> MSADSSPLVGSTPTGYGTLTIGTSIDPLSSSVSSVRLSGYCGSPWRVIGYHVVVWMMAGIPLLLFRWKPLWGVRLRLRPCNLAHAETLVIEIRDKEDSSWQLFTVQVQTEAIGEGSLEPSPQSQAEDGRSQAAVGAVPEGAWKDTAQLHKSEEAVSVGQKRVLRYYLFQGQRYIWIETQQAFYQVSLLDHGRSCDDVHRSRHGLSLQDQMVRKAIYGPNVISIPVKSYPQLLVDEALNPYYGFQAFSIALWLADHYYWYALCIFLISSISICLSLYKTRKQSQTLRDMVKLSMRVCVCRPGGEEEWVDSSELVPGDCLVLPQEGGLMPCDAALVAGECMVNESSLTGESIPVLKTALPEGLGPYCAETHRRHTLFCGTLILQARAYVGPHVLAVVTRTGFCTAKGGLVSSILHPRPINFKFYKHSMKFVAALSVLALLGTIYSIFILYRNRVPLNEIVIRALDLVTVVVPPALPAAM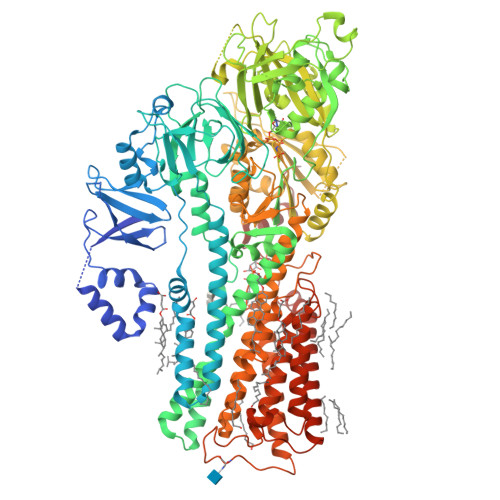TVCTLYAQSRLRRQGIFCIHPLRINLGGKLQLVCFDKTGTLTEDGLDVMGVVPLKGQAFLPLVPEPRRLPVGPLLRALATCHALSRLQDTPVGDPMDLKMVESTGWVLEEEPAADSAFGTQVLAVMRPPLWEPQLQAMEEPPVPVSVLHRFPFSSALQRMSVVVAWPGATQPEAYVKGSPELVAGLCNPETVPTDFAQMLQSYTAAGYRVVALASKPLPTVPSLEAAQQLTRDTVEGDLSLLGLLVMRNLLKPQTTPVIQALRRTRIRAVMVTGDNLQTAVTVARGCGMVAPQEHLIIVHATHPERGQPASLEFLPMESPTAVNGVKDPDQAASYTVEPDPRSRHLALSGPTFGIIVKHFPKLLPKVLVQGTVFARMAPEQKTELVCELQKLQYCVGMCGDGANDCGALKAADVGISLSQAEASVVSPFTSSMASIECVPMVIREGRCSLDTSFSVFKYMALYSLTQFISVLILYTINTNLGDLQFLAIDLVITTTVAVLMSRTGPALVLGRVRPPGALLSVPVLSSLLLQMVLVTGVQLGGYFLTLAQPWFVPLNRTVAAPDNLPNYENTVVFSLSSFQYLILAAAVSKGAPFRRPLYTNVPFLVALALLSSVLVGLVLVPGLLQGPLALRNITDTGFKLLLLGLVTLNFVGAFMLESVLDQCLPACLRRLRPKRASKKRFKQLERELAEQPWPPLPAGPLRSNSLEVFQ> MQNKTTASKSWVGTWATAPQLVEPRNMPPAPGLTNSTLRQVVCVSIGGKQLQFRFSNRFSKSPVTMKTVHIAVSKGGSEIEPSTSKELTFNGQPDVTMEPGKAVISDPISFNLKPRMLVAITISFGETSPDVTGHPGSRTTSYLLAGDQSSPDADFSQAVKTDHWYVINGIDLMAQKRAAAIAILGNSITDGRGSGTNKQDRWPDELALRLLKNKRTRDIGVLNMGIGGNCVLHGGLGPTALSRFNRDILKQHGVRWLIIFEGVNDIGGTPDKEAADKVAQGLIAAYDKMIDEAHAKGIKVYGGTITPIKKSFYYKDYRETARQTVNKWIRTSGHFDAVIDFDKAMRNPKDTLTLRPEAQSGDYLHPNELGYRIMAGAIDLSLFKE

Acetyl xylan esterases (AcXE) that target mono- or doubly acetylated Xylp are well characterized; however, the previously studied AcXE from Flavobacterium johnsoniae (FjoAcXE) was the first to remove the acetyl group from 2-O-MeGlcpA-3-O-acetyl-substituted Xylp units, yet structural characteristics of these enzymes remain unspecified. All homologs were confirmed to release acetate from 2-O-MeGlcpA-3-O-acetyl-substituted xylan, and the crystal structures point to key structural elements that might serve as defining features of this unclassified carbohydrate esterase family. Enzymes comprised two domains: N-terminal CBM domain and a C-terminal SGNH domain. In FjoAcXE and all studied homologs, the sequence motif around the catalytic serine is Gly-Asn-Ser-Ile (GNSI), which differs from other SGNH hydrolases.

Three crystal structures of AcXE from Prolixibacter bellariivorans (PbeAcXE) were also solved, including a native form (1.35 Å) and two complex structures, one with MeGlcpA-Xylp (to 1.26 Å) and another with acetate (1.13 Å). The sequence identity between the CspAcXE and PbeAcXE is 52.4%. Both comprise an N-terminal CBM-like domain consisting of three antiparallel β-sheets, and a C-terminal SGNH domain where the central β-sheet comprises five parallel β-strands flanked on both sides with α-helices. In both cases, the CBM-like and catalytic SGNH domains are tightly packed and connected through a loop of six to seven amino acids. The residues forming the CBM-like domains in PbeAcXE and CspAcXE are 1–175 and 1–176, respectively, whereas residues forming the SGNH domain in PbeAcXE and CspAcXE are 180–385 and 181–386, respectively. The first seven N-terminal residues of PbeAcXE and the first 10 residues of CspAcXE did not have electron density and so were not included in the final structures. The active site of PbeAcXE and CspAcXE is located at the C-terminal end of the central β-sheet of the SGNH domain, as is common for all α/β/α hydrolases. The Ser-Asp-His catalytic triad is formed by Ser188, Asp363, and His366 in PbeAcXE, and Ser189, Asp363, and His366 in CspAcXE. In PbeAcXE, the oxyanion hole that stabilized the oxyanion intermediate during catalysis is formed by the main chain amides of Ser188 and Gly228, and the amine side group of Asn265. The substrate-binding sites in PbeAcXE and CspAcXE are mainly shaped by five conserved loops, from which two belong to the CBM domain and three to the SGNH domain. As indicated by a structural similarity search against PDB using Dali, the structures of PbeAcXE and CspAcXE are most similar to structures of GDSL hydrolases of unknown specificity and some with esterase/lipase activity, i.e., TesA from E. coli and Pseudomonas aeruginosa.>MSLPIRNSIKRYKEQLKKPLFKNEALYQLTKLYLSLENEINENELDECKDYFNQLKQSGVLKESQKELKEITIDFQTITKQYDLAEQSLQSAIKSYPDNLNFLLKNINLLSINKKYYEFFKSIKDSKIKYQRDLKYLNFIIKQIDNVAIKAIKESVEEIQANTMLLNDSMSYLNLITLKTEILDYIIRATIHNNLVSSNSSGSIDDIDDIGDYYGNNNFNQKLTRQLKEFKKQVKKIRELVSLYKEPITLSPSLEEFNERYFFYKGILIDYEYSNISNITTSISNIKNRQNPPFKSYLKSLQKDITKSSSSNMLEPIVKLSSEVSRQLFYSINRIIGDGNEIDLKLNFYASLNNNINMNLNIGDSGMYKYLDYLVSKFNSVSSPNDTDQLDTLFIESIEKNDFQYLLNNPLEFQRFISFSLWHINKTSSYTTLICWLDKIFNKFINRINFELQQLSSKSSSSTTTTTTSSSSHITLLHIIVYCINLIFETDYQQDYQQQQKQQQQQQQQQSYQLSSLEVYLDSTLNVPFLRNSLPWKIWNSMIYYSNLKPSSKINSTEIFSITTLSELLNGILKNGDHLHPLTCYKIAKDLPMITQHYQNEVDLSQTDIDISKIQATYYLITLRHITYLNQQRQQQQQDNNNNNDINNNNNNNNQIIQDKNFLKNIENTCNHCLSDLYKDKQNLKGALQYLLKVDTPIAYVETIYLCRDIIYNNKSNPAYTRPVIQSLITLMNQVWNKCQDFNANDLDYYQVDHDEYLNDIDASLEIITKLKDQYNFYDVPSTPSSSSLYTTPTKPTTVVPFSSIYGNNYNNNNNNNNNSLISSTPQRGRLSLPSTSTPLKVSMLSNSPNKSNNNNNNNNKQIQQSQQNKSDLPKFNVVEEEEEEEEVDINSFKDVFLQRRKERAELLKTLSNKRKALVCPQEFNKPLRSLDYVPPEGTVITKPTVVPTTTTSPIQTNSAFFGTTTPNSLLVNPVVPLPTTSTSPPSLFGVTTTTTTTSPTSLFGKTNTSPSSIFGTTPTSTSTSTAPLFGTSAPTSSLFGTTASSTPSTTATPATPFSTTATSTPSTTTTPATPFSTTATTTPNIFGSTLTTGLFGTKTPTSVSLPQSISTPTLADKTIKTEESTTSVSPPPPPPLPTKSNTPTKPATITPTTSNATSSSSSMSSIFANASVNASSMFGNTSSSSSIFGTPSSQTFGSISSPTSNLGSLFGGTKDFKPVETTTITTATSPPSISENKSTTTSDTNKPVETTTTTTATSPPSISENKPITTSDTNKPVETTTSNTLFGATTTTTGLFGLTKTSNTATGISLFGNSSSILNSSLLSKKDGSSDEDSDEDSDEQDSEEDSEEEKGKTTKSNSSLQRKKNEVSHKKDSKNRLQTLKDKISKKNNNNNTQKDIIKPQQQKQQTSQSSKNLSDDDQDEEYESQEEDENQDDDQANEEYDEDDYEEEDEDYEEDEEDEDEEEEEEEDYKEDPNKPKPTFLFGTSSTTSNPAQTTTPTTSTPTPSSSIFGQPPTSSSVFGSKPTVFGSASSNSSSVFGQTTTKPSTGSSVFGQNSSSVFGQTTTPSSGTGVFGQNSSSVFGQTSTGTGVFGQNSSSIFGQSNGVMGSTSTPSSTSIFGVKKSDELTKKTEESVKKTEESASSTTPSKLIWKCLCCENENSEKEKSCSVCMVPVPKNVKFESPASESNTKPSLIAPTAFGSNVTQTSTPLGKLIWKCLCCETENLEKETSCSVCMVPLPKNVKFESPASESNNKPSSLFAPTAFGGNAPPTTSTAVESSKLFGGGGITFNAPNIFGNNSNPSNLFGSGNNNSSSLFGGNSTTNPPPLFGNKSDVKTEESEKKAEASTPSPSTTSGKLIWKCLCCETENSEKEKSCSVCMVPVPKNVKFESPASESNTKSSLFAPTAFGGNAPPTTSTAVESSRLFGGGGGNGITFNAPNIFGNNNNPSNLFGNGNNNSSSLFGGNSTTNPPPLFGNKSDVKIQESEKKAEESEKKANESTPSPSTSTPSGKLIWKCLCCETENSEKEKSCSVCMVPVPKNVKFESPASESNTKSSLFAPTAFGGNAPPTSTAVDSSKLFGGGGGGSNTITFNAPNIFGNNNNNTSNLFGSGNSTSTPLFGTKPTETKAEVKAESKTESNVEETAPSSTSTPSGKLIWKCLCCETENSEKEKSCSVCMVPLPKNVKFESPASESNTKPSSLFAPTAFGGNAPPTSTAVESSKLFGGGGGNTFNAPNLFGNNNTSNLFGSGNSTSTPLFGTKQTEIKTEVKAESKIESKVEETAPSSTSTPSGKLIWKCLCCETENSEKEKSCSVCMVPLPKNVKFESPASESNTKPSSIFAPTAFGGNAPPTTSTAVDSSKLFGGGGSNTITFNAPTLFGNNNNSNPSNLFGSGNNNSSSLFGGNSTTIQPSQSLFGTKSTETKSDDPMSLKEMSNTIQDNDDQNSDSESHEELESGSEEEEEQQQQPKVTLLSSSFTPPSFAPPSFAPSSFAPSSFAPPSFAPPSFAPSSFAPSSFAPPSFAPPKPENTSTPTSSIFGSFSSQPSGGGISAFGPVSSNSSSPFGSGFGSASIPSFGQSQVNPLTINPTSTSPTAVFGGSTTSQFSSSSPAPIFGSTATIKTFGDLSKPSLSNNENKDQTSSSPSKPSPSPSNPTFESINKEKESVEDKNQEKDELKDEKDELKDENEKKDENEKKEETVESDKEKEKEETLEETKQSIESDKKEEKKEEKLEEIVQSDKEKEKEETLEETKQSIESDKKEDEKEEKLEEIVESDKEKEKEETLEETKQSIESDKKEDEKEEKLEEIVQSDKEKEKEETLEEIKQSIESESDKKEDEMEKVFSRIEETIKPNFFSTKEDEEEKGDELKDEKDENENEIESDNEKEKEETLEETKQSIESDKKEDEKEETLEEIVQSDKEKEKEETLEETKQPIETDKKEDEKENETEPEKHIDNEKKDENEKKNEDEKKEEETVESDQEKEKEETKQSIESESDKKEDEMEKEFSRIEETIKPNFFSTNKDEKDQETKEDNGNSDNNIDQETKENEKASKEIQDEEEEKEKEQEEPNLSLLSMDPVRCMSLSGLPIFDQTVKVEEEIEYEKDDGDDDDDDETIEKDSSSTTTSTTTTSTTTASTLTPQKPLFAPSSFAPPSFSLPTPTIQASSIFGSFSSQPSGGGISAFGPVSSNSSSSPFGSAFGSSFGSTTIPSFGQSQVNPLTINPTSTSPTPVFGGSTTSQFSSSSPAPIFGSTATIKTFGDLSKSSSSNNENKDQPSSSPSPSKPTSESTTKEEKVDIVEDKTDKIEENKEDSEDEKVITEDTNNQSEIKVEENKEENKEENKEENKEENKEEEKEEEKRIKQQQQSIESESDKRENEMEDKFSKIEELVKPDFIPCKVEEKLSEEQTKENIDNNDDNNTTSSIVVQENTTETISENDNDQSIQLDSNKQEIKKSIESESDKKEEVMEKNFTEIENLVKPNLMNSTQEEQQNQENKVEKEEENVNKTEEKEEDENLEKQNQTIEKENEEISELKDIQENNENNEESSTSSDGEESKSIKDVDTSYDDVD[2x];>[8x]MIIINKNNDKKSLFLLLVSLIFVLFVSNVIADTDYAISPVSLLLPYSTSKYRKPYKLEANKGCFEWINTNPDLVEITPLYESAASCSPSSNDKQQNIGAPDLSLWDNSLNQPNKKCSKAVLVSVRSGTVSERNSAFIYAEEQVTGKKLQCEVFVDRISSIVIETTTKTMYKDDLEELHVRAYDSVGNVFSSIIGLEFEWSITSGNIIQIVPFRGFPLDDVALKMEQESLQTSFVLVQGVDTGRTEINTKLTEPTYKDIQHSTTISILEPLQLNPSYLLYVIPGTQIQYQLLTKKRNILENIPLPNPNYIWSSSNSKVGKVDNSGNFMALDLGRTDLKVQHKNMSDNKVQAFVNVVHPSYLAIKIEPLKSGLGPVSNWNLIENRDYILVVELYDASGHKIHSSEITFDLNIPTEYFERLPSSQIPPNTPKRSDTFYLKAIKQGLVALKASLVKVYDLNLKKYTQLLNPISVEQEVTIHSQIQLSPPIVYLPYLPNHRQYSMIRPIGGSGEYNWYTNNSAIVTVDPTGAITSQTSSGQTEVIVVDKKNPHNRDKVLVIVLQPDEIIITPSQVEVQVGQTLKLSTQLLSKQLSKGVHFDSCNLDDLEWRVDDSNANNDNNGGGGSNQERSFSLLPLQKTNTPKKEQPDLCSTREFLAIKEGSNVISVSYMGMRAKILIFAYPPLKSDQSEILLTLGSTLNVFFSGGPEPWHLERKSHFQSIVSNLTNEQNVLSIVPGNGNSFRVTCLTHTNPSKPIGIELTIGNKVTTTNPYPASPSITIPYSCRPPASIQLQVANLPKDHQIQDSSHHQQIQQQEQQQQQQQQQSTCQDTIFSIKKQKQGEIGTYKIRNDRDIPFIAQVFDDNGKPFTNYSSLVFDWKSSDQTQAKWLRDYNQNDHLSTLSLSKEQGKVIITVSILGYDQELLRQNKIRSSDLDTSKLVSSLELHLLSSVVLFPDYYTMYLNDKNHLKIEAIGGSKNFAFTSNNSKIASLSYQPNSDFVTVIPNQQGYLKVEVRDICLGSDNNKDQQQQYQQKQQKHQQQQQSNTSPSIVQISEVHSIELDVQDMVQVGDSINLIVKGFSQNGQQFDSTQYQYMNIIPHIDNPNVLSMTQSSDSQVFTLKGLDQGLVTLSVTIQNPKTSFSATSKTIQIQVFPPFRVSPSVLHLVPGGHFQIHWTGGAPIRQDVSFVSSDPSIVNLSGREDLVGELVALKVGEATIKAIAQIVDPITGKKTIIGEDKLMVYVKNMTGIRIHSSINKILVGNEAKLRVVGANGETPFTYGTVDLFFKWECLDSNIATLLPIYERANTTVEAEGSFSVRVMGKNAGSTSITVWAYSGGDKTKHLFQAASLQINVIPDIPIQTTSLLLPLNTPSSFIVNNHLDKTGIEFYPLMDGHGSSSCKDVIDIGDNKIVSLDKIGTCYVSAVRDGRMDTSKLFKINSKPFSHLELLPINPTSTVIPIGGSMSFAIYLRDDIGEVFTEYGSSAIFSSEVSNTGIISSSIDANVVTIKGIRAGLVTLHVYLKDMPHLDDYIKIFVGRLVEPHQPILHVGSMITFSIAKDQLEQRGFSLPSSDEKVWSSGDPSILQVDPITGKATAIAAGTTTINYIRNPSSQTQVVISKIGRIKVDFSDQIINNSKKRYEYNLKFFTAGSDIELSQDSTIDQNIKGICTIKESTFATAFFEKVKGKEQYRCVVQPSGVATSSIDKVTLYVEVSNAHKTYQYDTTINLPFESTFSIINVRDNKIQLSPRQSTFILNIQSSSPIFVESSDNSLLSVQQISSSGGDDQLNNLYKYAIQPMSVSTSFQNVPLLISSADGKSKTTVTVSYSKSGSTTSDQNTSYVESSTINSHPFLFSFIIIVGTLLIGLYASKKHNDKPRVYINPNSNLQTSSISSPYRTPPPHSFTSPNRSTYGSSSIYLNN;>MIEEHNCFEEFINTAAIGEQQVYGEYKSKLDSFTDESKLPYELLLERKNLVELKISDEEYKKSESALKTPNPTLLQKFQINFYQTIESINQVFKPSSSSSNQSSSSSSSNEDDSLQNKKIKVMSWHPQHRLLAVCNKNDVIYIYYFPNQDMYGMGNVRPLTLWFELQSKVYDIQWKPFLPYTLAVACENGIILWEIDISDLKVELKRTSPNYRINQSSTCANILNYPYFLSNTITWSSNGLQLACGSTNHSSILLWDVVSRVPTFIPRYNGNSLLVWSPKNDYLLSCGGKTCRIFDISKWDYNNKEWPMLTNYQTGSWNGKGEYLAVASGDRIQFIQCINRAFESGGELMYVEKTSTYRLQNVGGSGGGSSSSELFLGGHIKKIAWSPDSQRLAVIFYLNSKSRNNDTYCAIYKIKTYPKFSVTPRGFIRSKDQSIQSVSFVPNYKKGSLLSIAYNDGTIKFFPLLYQYKQ[2x];>[6x]MNVKEMDFNDLSNKSNQIINRISSFSSPIGLSSFNIERNLQEIGDTSKQLNDLTSSKTPFSNPLEPNVFQDSKINRKYGLDPKVLAKNLSNINTSSFTDVQSVPTDIDGYLKVQFENIILNTICDIQKKTSKEFQSHYEQTSIHDWNRDKKYLEEILGQKHIKVLPSVGGASASNQSSSSSSLFQQSVRGGLSSSIMGQSVRPTYGQQSQFGGSSTISIGGNISRVGGGSGGGIYSQRQTGQNEDRTKLSDKMKKYASIIEEYDIHMADQSKSYGFPLVHRLMDACLSTDINIGGGINTNTATTIVTHVWNLLLTLTSEIDTTNYIQQLKEQQQQQQQQTPQLKEQQQKQQQLTELQKHTKYHTKPTMAQLLKRSISFLETQFSQVIESRLPKHSNVSLPLNIIVAYIKSLNQSPLTDSSDEIYEGCSIWCIIYYLLRSGYTLEAYQFALEKCGSRYFDILSPIFKEKQQQQQQQQQQQQQQQQQQQQKSSLPTTTNNTSINKDQRDRMTREFNTAKTESKDVFKISVFNLLSCNDPNSTKQQVITSIQDYIWWRLNFIRERITIEPTNDSAISLLESLQNDIKNSIEKNRNNYETLEIFQLLLVSLQFEDAIVSLYQFCPDDSLHLAIALDYYKLLRTSNSGINNKHVDEINKFNKSTTNTNTMTYQQNQQQQQQQQQQQQQEQQKEIYDQTSKSIHLVEMIKQYTKIFSFEENREAFFYYLLIADNDIKIQEISELVVSSPNGFKFAHELSLFSEFINKQQWRTIIEQSALELENKNEYQSAIEFWIMIEEYPRVLEIYNSRISVLLTSISSERDQLYQFGKQLFNDYQGRLKTTSTARTSYLAFEQLLKLCDFFDLYNKEKYQEAIQKIENLEILPISESEIDSKVQDYRFLSPHITRNFSSIIQAYVDIIVKQYHLLNNFDEFTNRSALFAGRKQTIQDLQSRTQCIALFAGKIDFPMSGNILPRLMNLFISMSN;>MSNTGGNGNDNAAPSLSTTTENVNGNDDTPSSNLTINDLGGSKFPPQPKKSKQQQQQNITDRLSTFSNFFEDEKLDKDDMKLEFDKIEKKLCDIFETDTIPNNASKDQITSGKIKIKGEEITISKEAQDFTLELSSLLNLDQILTFILIREYLTNNNNKVLNYDKSELFNLLDYYYNERASLLCILGSIIKKESSQSKYSSFLKPFIEKNRASIESRLLSYLISFYNFTIPSNLEELQQFYCSSIIKEQLIIVETLFSYNYLKVKKSGNCSNSSSNMNDVNELLIILKKINQLQIGSYSDQLIGILNSMKRNSEVIQWLKRIEYVLVLLVFCNNRDLLRHESLQQNELEIINTITTLSQSIHYNAPLATSLFFTIINLFISTSSSSSSSSPSSSSSVNFSNSLQQYFTKASSQYDPIDYIFNCLSNGFNDSTYLAGYCDCIHIFLNRFSEVISLTDVSEQHVDRIIDIYCMLHEKGGEVLSSILWSERSNDPVYQFSISPDCLNRNPDRVLSILKSIIINDTSSQAVFNELILININNQSSSKQIISFNDFNKVKEVLDITNDDGNGTISGVMKRDIISQSFRLYKSQFKSFSVINDGSGGDGGIEIVFTLHDLIIDLVAIEFNSFLDSLGQQAFFDQRTIEVSKAYIVVLDLISKLVNFTPDSYSKYFWQLFENNRILESIIQVYLRLCNQQNFTVNSIPTNINIKESNGNGGFQQKINKQQQQQPTLMSSYSTAHYNFNIITNVITSILSLFTSFSKMNPLPILNLLIEKGIWSSSPTVLISLFKRGSFNHLYDVEKRSSTTSSTSSTSSSSLSSSTFPLTKSIVKLFNTFINPLNQFEKCIDRSQYIGYLESFISFHLQVISDYPIISGNNNHNETWEMISEIFSALDFILNKSQSRNSILKSLAFKIICSFSGGILQCTLSSLLDLEVLQNTNKSIDRTSSIDNILKSSLKFSKSILSTIYLSIVLKRSNKINNNNQNNDNNNENNNNNNNGDNNNNNNNNENNNNNENNDNINDNNIENYENEYSNNLVEQFLTTFFIVKQNETNLLIDQEDRNGLTSTIVTNSITTETITSKTDYNNLFIVLFNYINIISDCQDIQILSCEILSSLVRILRVLESNFSVSTLFNTDEPFILMIEKFSKKFIINNNEFDVWSLQLKTNILRLLVESSTNQIYFINRLLNCENNNINNNNNNNDDSGGDKKNKSFIIKLLLDRNVSINDNSEFSLALFQLVNNLYCNSIYYDSFVDQLNNTQDFWNLLLDMQKTINEEEEQEEESIINEELICKKLKITYAIEILSLSVLLSSDITTATTTVGNLVCSTLSNNKWNEIFKNNKSGIVNMINNYYFQFIDLENVFPIQKIRDYWMVNNLPSPDQLQTTIAYQYFPNINNNIPIVELFAIDTIIETSKQFNDQYYLELLIQRNLFELLTTTNLCLSRAFSKLFRVILMKQPQNFININGGSGSGSGSSNSGVPLSTILHTLVDKATSIENQSIKTLVVRNDILMFLCESISTASHLWCKSCPIESVDIEILSKLSNLLAQCSSNPILGHSISYHILTSILILVENTSQHQYIEIKVFNQLINTLSLFITEPHFRVPPISSMDGTTTTTTSGGNVGEGKTINGKQKKPLPSICNLSIYLLQVLIDRLDPNALIAAFPNNLLENLAKLLKNSLNMVNGNQIDNITASSVLNLLISFCKQPLVSEQLLDNRIIQLLSDHSLKYLQFSMDPYLASTEISAATASIYGGINYYFHNNDDDYDNHRQFNQKKNKWHRVWTLVIKFLISVSKPLESSERFIEQLSNFILSHKDRLFYYFDLFNEFGATQHSQYFTKQWFQQLEYITSLFSIFTKYTKRYYLSMNIYREFLSLAYRLLVSISIQCSELNFIENNFIPITKNEKHKNLVQVKEFIDDSQRLQQQQLQQQQQLQQSQLQQSTPYRTSHYQQQLLQLQQQLQKQQQPQQQNIQNSFFKFSIESNYTHIINNCFTILIRINEYVRSSNEFVPQLTIYPNVATFGTFGQLSQYIISKLFQISNVVDKLSRNNNNNNNNNNNNNSSSIYNNLEDQNSISVDELLDLNLYKTKIKQTLEKNTLLLILYAKQTPPSTSPQETLRENQVNNIITHLLKQQFNNNNNNNNFSQNRTPLKNNNNNLNNNNTSENDENDEFLNFLSDLQRVK[2x];>MEFINSFNLVMSNIFDNHNNSSIEFWRICEQINYFQNLWFRIHDDLIISSFKLMGSLARCNTNEVFNFFAQGSAQFTWAKLFQNFSSYAHALNSIEFSQSIQSNQMNSSTTTTQQISSTPQQHQQHQQQQQQQQGYNNQQIPNTPYQQFQPTMQYQGQQSSMQQSVGQQQQPQQQPQQQNTPNTPNSTTSSNTANTTSPVKITQLLLSEKDSDALSSIFQLISRLVESSMAVGNVFLKIGPLISLAFQFAVSQVDSKLKSSALSVITSYSQYPIYVADIWRLINETNLFNSGLSAIGGLNELSFTQQSLELLLQLIQQSSFLFDKSNHYQESLKLKSYLDSCMDLFNLLNIKSFNTLDEKWKFALTLMKIFEFSIIQFNQSIQNFQIDKQHPCYQLYIELNRSSLSSNLYQQQQQQQNKYQQQQQQQQQSKKTTLENIIKIIDYSNDQSILIQQQIQQQQQQQQQGYNQDSSRVILNLVFQQLQQQDNDDFNLLVLKCLDLLLLISDNTVYDIENAKSLVVNLSNMDYSRPIVSIAKLIDHELPAISLRAIRLIYSFECYTHQISTVFLDSDPNLILSKFIKMMEFNESNFEDFSGTNYDQTISFIRYASNSVQWTIAQLIMLCLSNISSGRYTLAHFLLGCSSNLDLSKDFIPNSKSCLTLIIKNVMNSQFVERYPHLVDCYHEIIWKMSSDPITWKPMIKYIQEEFPNYYHDSLLILRNAITINGSSERRTEALISSMSWVFKTCSISIQNSYSIEMKQFLTRLIFPSLMNLNQPSMNGGIGGLNGTINNGLIMGISPINILSLYNTIEFQLPEINRPRIFSMYPNLIEYFTTNININNLNSNNNNNNNNNNNNNNNNNNNNNNNNNNNNNNNNNNNNNNNNITNGGTSQLLDIIKIREVLKNDFNRFSNEFEIERELEECCLINSSIQLYNSKLKALDGWKSFINISLAQNTIEIDTLDESLLLSLLQRIVIDFSNERNPIESTLSIGYTILTILFTLKLKKDSYQLFINSSLTTNSTDSNVIEQKMKSIFEGLLQTVLKSPHQAIRGISYTCLIQYLDLSATTPTTPSLSPLSTSINNVVEMNNKSKNKNNQDKEQGYGNLNIGLIISKIEDKFIRILSSDCNSFSRGWRITAISCMQSILSIDNLCGHRSLMFLQNKGFIINMINDTCSKYLSDNWENIDPKDLHVYKSQMSLLLKISQQMDGVHLLMNNNVIGSFVKSPFLNYIPTDKIFGKFIEILLPILQLFASLCCYCNNTSKNNGNINNNNNVGGTVLIGSDRNEIYQELFDFLSNHSDLFIIILSDQSSFSHPTLSSLKVLKLTCFLFSKVSSLFFKKSTTTSSSTSTTSSHNRTQFNRFHYCLINLLVKYSVNSKQIIELVKPENIDEELLTEKIDFSYLPKSSIENQFKNIPDDINIGGVNIGLTSKNSNNNNNNNNNNNGSINGKKSKRKNQFQILIKETITSIIHDLLLYCRKVSIVQDSNFGFVCFNSNLNIYQQFQSFSSLRSTNRNNSNNNNINNNNNNNSNNNYNNNSMNSDMDNDDDNIINNNSYKFNNKNNNNNNDNNNQNKNSIFGGFGVNNSIINGNNNNNNGNNNNNNGNNGVNILPSIDLAINILVDNILQYSFYKVDLSQCFKLLQSYDQLTNYQYQEILQTGEDYPAFGPTQRNHMVENILKEKIIDIETQISIIHENIEILLLLIVSHSFYFCNSLYLLFQNSNNNFYSSAIGGTISPTLASSAYYPTTQQQQQQQQQGGSNLKITDLNASTTTSNIKKNNESAFLSSKTNQNSGGMLSSVFSYFKGQQNNTPSAQVSQIPINSTPYSTNYATPHQHQQLLQQQQQRQQQIQQQINQTPSNELSPQEIEVFLKRLKQSIFEREVNQLGGKLSDVILNQIDKKSTLIDLLLKKLQDLTK[4x];>[4x]MRQSQLYPNLGYNNQNGQFNYLPSPEQQSIYRNNIQTPTSGISNNLFPLQSQQRIIQPQYHYQTPLINNNIINNNNNINNNNIVYQQDQQTQPQAQPQQQPQQTQTQSPSQQEKEQEQQQQELKEQQQKQQQQQEQEQQELMRQKKTNSLLSITPFNKEEDLKKIFLNSIESIDSSIDKVATIPDPTLKVLYKRDPGFNYFDGGSYFWSTLVIEKHIELPQEITNGYLSTSTKSLLGLFPEIGRAWISIDQTLYLWDYRDSGELISHNLSQIITNCALIQPKKNTFKDAVKKVMVVCTHVEIFLFALCYSNETKFEILSTLSIPSDNIFITDIVGTKEGRIFLSGQDGNIYEIEYSKDNLFWFSNEKIKKINLTQTFFNSFINLSKKKEIIQLIYDEDRYLLYSLSKDSTINVYSLGKIGDKFEHLKTIYPINDIDSLFNNNINNNNNNNNYYSQQYQYQQQQQNQQYQQSQYGQQQQQQQPNQYGQQQQQQQPLQQQQQQQQQQQQNFSRKNMVIMSIHISPKETEFNFIAILSSGERLYYTLNRLAYIRSPPNNVDNNGNSNIHYTYYSNGVFFTASEVSDQEDRLVGTTLFGNDIIKSHYETSKSGFSNQISQDTLSEKSNLFSIRGRVSVIKEDIVNDGKPTVYYKELSNEHMNTPRRFLCLNSLGLHFISKLRYVDLLQNILSSNNPQDIDNFFDAFGKIIASSLCISLYCSSPHSSILLHDQVYSGISIPKTTTTRIADLAMTFLRRKSGKPQYYQPVVIQQMFGDMGAPVNKTELMYSNAYNGLLAYLARVLYPLWNQSVVTSAGCSYWSIVQLQLFQSHLSNLLSFLDISQLIPKGQEIPIIKIATNKTSSTTTTTTTANNSSSNEIYGEDEAIKNEKRSLIGLKNIIVKSIQILNLFLILSQYNFKQLFDSSSIELDIKRKIDLLKFRDILNSDILGKNLPLPTISSLTTSTTTTTTTTTTSTTSSSSSSTSPLTTSTSNSTLTLLIDSLMKTLNSHNINIDQVSNQLETECPIFFKKENRELYKVKEKLNMVLRDGSTYFTDSLVKDSALILDSISPNYNLSEIVDLFIAIKAFNYVTPLCLQYAQDLDPRGITLIPSNNPSDEFKLKLSQKKSTFQEIIKLLNFIQSDNNNNNNNSGGGGGDNNNYNNTFEIIDIIIQQVLVCQDRLAHEMIYSWILNNGMTSKFFEINTPFITEFLFANDIDLCWKVLAKHQELLKAVHVLFQIAERSTTLDEKILAYTNCTMILSEQKDEDAYIQAKNQITFANIQKQIVLQLENYLNNPNESNNRNNSSNNNGGQPFDINQIKESISNLNKTIFDITTLFTDYARKYYLHEQMLYLCHIGNHSDQNFIQILWKIIIDKEIPPPSSNLSLDDNAENDDGLKISVGGVIESLVSKISNIGYDFYPNEITFPVEFIINYGERAIFNFSRNKSEAEKKEISPNWLTSSLHDHVKIDYWILVDYYNNTIEKGSWKEEDESLIYITSVYFYLVESLINTIQTATERRLFSSKQILQSLENRESTFKSIFNRQRSSLNQETIKKLEQLLIKFEKIISISKSFKDFRGY;>MQSQPQQLQQQQLQQQQLLQQSQLLQPQYFEKQQIADYIDKTFEKKIKEWKTWTFSSVFIIFLPLLLFQMLFLSFMFSPSPKSTSTSMISVILRTTGNHIFGIILYVIGQLILGASYHSICSVYRQVPASFKEQFTVLSIPHLIFITLNTLIQPLFLYFFFSIPLNKFSLSSIIEVCYQDFSETIPVAKCELEYNLFFYLFVLSCIGLVCSGLFRIYSNQEFVYSFPKANIPTFIQIKSMLYNNFWISFYTSFYLFFLGSFLLGILFLILFKTFTIQILIFSIKLWCFTFAIIFQNLTRNRLFEIYFTRGLRFTLETFNSVTFDSSNSQQQQQQQQQPQQQQQQQQQTLFDNKPIIENGSIFLLKAIYSCDPLIQALGWKDFLHLSKYSQPRRTYLYREMSELLDQPSILKIIRQYEDQINDLSLKLSCPREYYESLNSGNIKKEDDKNKNSNNNNNNNNNNNNNNNNNNNNNNSNNNNNSIIFKIGNNIEKIIKKTLNFISGVKFDYNLYECEIRQALSNTQSILWSIESIGSLIVSAQINDDRETMELLHRYQIPQKFLIPLFQILALIDQLEKDLSHQIELDKFTINRDYYFLKSFSNLIEPPLNCLGILKTSRPHFRIFKLVGKNMISQVLETIGHQISDISFPYDLRTTLNSYRNGEFSIYQ[2x];>[4x]NDLLSIPVNSIYEEKYDKRWLTVFGFSHDKTDLIVDELSKYGNIIEIEYPQQPNCNWIYLKFESEYSSIDLLKKNGLILGNCMIGIVPCKEKIRN;>MSLFGNTTTGGGGLFGNTTTPTQTTGGGLFGNTTTGGGLFGNTATPTTGGGGLFGNTATPTLTTGGGGGLFGNTTAPTTGGGGLFGNTPTQTTGGGLFGNTATGGGGLFGNTQQQQQQQQQQQQQQQQQQQQQPSTSLFSQSSLGSQSSLGSQSSLGSQSSLGSQSSLGSFGQTQQPQTSSLFGNLQQQQQLQQPQRSIIEQKLYDFMQSISPNSLNCRFLYWFYNYQANGQLVDPNSIPKPPNVTVDQWAYALSNNPDPSILIPVAAKSFDDLINRRMKQEETIIALDQNTQEALKRMRDLENHLNFHIHTQLEMMRKKQIELIQRYIEVWSNLEIYQSKGKTFTTSEERIMKKIYELFEEINQPNSIKSKVEEISNQLKLGSMEKEKIKYEISPEAVEPLYNLLKNMTISIERITNELEIAVKDAQILKNELYQLKKC[4x];>MFQTSGLFGQASTTTGGGLFGTAVTPTSTGGSGLFGTSTSIAPTSTGGGLFGTSTAVTPTSTGGGGLFGTSTAVAPTSTGGGGLFGGGGGGGLTSSIGPQGGGGLFGSTTLPTSTSGSGLFGGQSSIGFGQPNSGSGSVSGGLFGSTSVQQPQQQQQQPQQPLITESTKFSDLPPQLKNELQILNKMIINNNSLMNSFSNYDTKINEISIGLDQVASVMDNLFNNFDIHIQSFKYLEESLAKPLNSVNEQVHLLSTQFHSPFSQARPSKEMEIIVDSLVEKIDRIKQTILCVTPTNKSQSQNLSFQESFISTLQSNQIILRNLAYIVDNLVTELERHKKHFLLYKKKYYNQNYNPFLKQPKLNEKTDYHGSSSLHHSHFSQSSNLLSSQSSLFGSSMYGRQSQQQQQQQNPQQSQYLQSSTFQPIQTSTSFFNPTSTTTTTSFGLTNNNNNNNSLASNNSSGGSSGSSLGSLGSLGSGSGSGLFGSTATNNSLGSTSSSGSTSSSIGGSNSIVIPPLAIGSITNNNSGGGLFGSSNSSSNSLNSLSTSSSNLFGPPQTPTLSGQGSTLGSVVFQSLVQLQI[4x];>MSNNLFGTGSSTSSSLFGSTPSAGGLFGGGSSTTPATGGGGLFGGASTTPATGGGLFGGASTTPATGGGLFGGASTTPATGGGGLFGGSSTTAPATGGGGLFGGSTTTAPATTGGLFGGSSTTAPSTTTGGLFGGSSTTTPSITTTGGLFGGASTTAPSTTTGGLFGATTPATTATTTTGGLFGGSTTTPSLTSGGGLFGATTPAATTTTTSSAIPSLTSGGGLFGGSTTTPSLTSGGLFGATTPAATTTTSTTTPSLTSGGLFGATTPSTTGGLFGASTTTTTTPSTTSTTTPSTTTGGLFGATTPATTTTSGGLFGASTTTPSTTGGLFGVSTTTPSTTSATTPTTTTTGGLFGAATTSATTPSTTTTTTTTTPTTGLFGSSTTPSTTTSGGLFGSSTTPSTTTTTTTATTPTTGGLFGSSTTPSTTTTSGGLFGSSATPSTTSSGGLFGATTTSATTTTTTPTTTSGGLFGTSSTTTTTTTPAAVAATSSNPLTTSMLGGSSTTPNPVSASLNNSDPIGINESKLLEQLLNEWVSEIENQTKNFYDQAKTIFVWDQRIMDNSQKLGKLMDVVVKLNSQQNALNQCIDVVRDQQALLERSLNALDSKIKSSPKDNETTADLERERIYSLATKIDDDIIKVENKLLGVVNKINQNQVKDDNPKDLNQKVSKILNDHLNTLQWIDKSTNILQESLKVIESTSLPETSRR[6x];>MYYSSSKPIKKKPNTGISEFNPTQSQIQQQSCNYKITPTYDLPFILTQAINDENQQHQIEQDLTGSLSSRDGTCFIIYSNELFIWTIDKPQYCDRIELPIKQNITRQHIVVYKNKSSSERFSVFLCSPLTGYIRFWGNSSKPNVSQDLPLENPGNNNNFKIFITECQPFGVIVGNSLGSIYLVSVKNNNNLISKKINKSQGMLSYLYLSRQSPVISVFSSPINQQQLQNNNNSHHHHHHHSTTLSSNNFSTIPSRFIYILTEGSLLKYEIENGTERIILDFPIQKEITKLFSNFPKFHQMNIDTIIDQNKDEIQIVNFILYETSASQNLVKYYILQIEIQDDQVLRIKRLDSFSANKKLGGGVTSIEPILQTNSLKYYLTWFDNIYYYSNGGGGGGGVNGIISGSISFQSDIAFSGFYKNQFYFFSEQGINKLDIQPFGSGQLASSELHIQDTIKNIESDIYMDTDNTTSVTGTPATTASATISTTPTIVSPILFDIPKDENLIGSKRNNVLKLMNSFSLKQHTRVDQFVKICKGYNDFDQVIQQVSLWIIDQQPNSKFWAEDGKLLHMFVKEISVQLNQQLEDKKKRHNFLLTCIKDTDLDKLLTTQTKEILKKNEIKIKCAIELRNYQNQQEQSRKSLNYTTTTTTIMKGASSSSSIFSQLIESLVAERNPNWTNIGMNVFELFYSNVSGIDQILINITSKLQELLQNQPQQQQLLTSANKAQILLENCELFYLISSSFPVEYLNSPIIQSTSISIHNLFPKVIQSILNFIQLEFPNQVAGLLGGGGIGGLGNGHSSSSSTILFKKDLGIPNVDKQLYDHLYKLTEKYLYSLKINQFEQFNQFKTKLIEPFVECFKFQEAITLANQFDDFFTLINVYCYQQHQLQNSTITIATTITPADNNKLLIDCLNKFEKIGQLSKVYEYMLERDLKSELLQLPSDFNDSLFRFLQSNSELSWIHSIRMKNWTNVSNTLYQKSISNQHHQQQQQQQQHQVMTLKEKQKLLSLSKVSLMVSTATSSSSSSSSLELQLQPSQQIQLDVINQNLSLIKSQKFFLPDLKNVLSVSEVVQLILQREIGDEDPMVNFVSCIEIISESPLLLKKEEVKELLKLILELSIVNETVFFEKSISDIQLSYSLKETKFYNLISHPHFPKEIALVLLSPIIEDFYKTHINSNKFSSLDDKRQFEISVARLLELSKLEIGQKQI[4x];>[4x]MSENFKWNLGNNLNSNNNDDFFSTQPFNNNNKFDFSILPDDNNEDEFSGIVNNNNNMNNNNTLVKGDGGIFGNTQINFNNNNNNNNQFGNSLFGNTINNNNNNMEVNNDNDNNNNEQEFEMDNQQLQNNQMEMEEDENQFNNIFNDKSRTDDTIYHNTLEYELQPKLNDDPHLIPIELSDTFLKLSQAKINSINDDESNKLFYMQNNRKQKEQQLKNYQMEKDTWSILKKLYEYRDIQRSIDQKEKIDISQPNQVQVYNYLIKKDHKLRENLILLEWLEEMSSQVELNDNDAVFWEYTLIKLKKSNSITMLTNNQMVSELDPDAMSRQNKPIDKDDEKNQSRFLKTVWSFLRAGDRVGAAEYCTNVGQFWRAQTLIGLNYYQGEHSIGNPYFNLWKSNCLNISKNSNDQYERAIYGLLCGNLEATLPIQKNWYDYFWCYLRVLYDESLYRELKPYRSPLSIEEDIDSPPSTCISQINTPKDILEILKNNTSQIEIKNQSENPYHQIQELIIADDYSILFNSLPNLLLKNKTPEFNRFAVLLILFFRKREQYELISTSEDCPENIVINEYVQHLINSQQYELVALYTSLLNNESLQVDVYSRFLVNIIDPNQRQQLLVLAEKFGLNTQEIAQSVVKTITSGSINTTSNSFENLEFTGFATTINKNKQPKNKSTTTTKASTTETTTNTNTTTTPNLTNTIINQDSSITTQDDLVKINSIQWLCFEKQLLIKAILQSNLLLRDFISLNKYGAASELLKSLPKDIVMIAKQQSPLNESDTNNIIKEFRDWENYITANIRINLWLQNYSNQPKISNYLPQSLNNNNNYINNNNNSFNNIINNSIINSSIAFRLRGNESYAEKLDIERRKKEYDDVYGQWNQNNINFGKEAIVSIRSIIKTGWLCPLENQIGLFSEDDQSGHEVTLIRKKCIPSLFKSLYTILVGIGSIQKSSQLCNQIANERFRWYSIFSKKELQEILQLVRESSIKLLN;>SKYSAPDFDEDDQQMQQQTQQKQQQTQPSKVTFQQPSTKLTKPKFTANLDNFDSDSETSSGDENQDEMVPQKKTPFIKRVSNRESGLFDTPSVVPMSE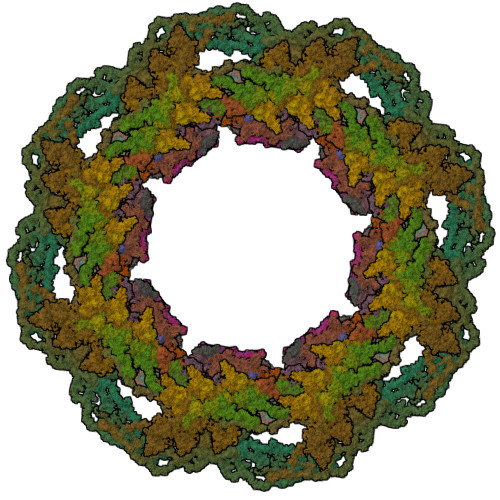KIETTPSKIARVSEPTSQSSRMSNNALKFSTFNPQQQQLQSSRFKSTGLSILSNPVKNLIQSDVNNEQSMFSNTTTTSTTRIQPLPSQQHLVQPIPTTISLNKNYFSKVRIDPQVYDRIVPKEESITNQYRMKNERLNHSTQDVSLFMRRSFRVGWAPGGKLISITKSSFKNLLIKKLPTDTKEDKKESIIKFLKNHHSHSSLVPENLKSIGWFSISNVQEQIESQLTLNVPSSQSVYYNRIWSLISNLWGNVLKGNGSKYINTNYSEDTIRKLNLNQWLKDVIAPLLRDEMDSLRKKTNSNYLEQIFSYLSAKQIKEASDLANENKDFRLATMMSQIWSSSESGKELILKQLTTYHSNGSDEFINEKRLEILHLIAGSVNKIYKNLNDWIRCFAVSFWFKYSLEYSIEDSVENFERSFNAHRSVYPLPPYLIKSTSTNSKQIEEQQHYYDICFLLLKLFAVNRGSSHFDKFKNIFYPENIGQDLLDYHLSWNLYTVLKSIPSLNKQPDLVNASNLHSSFALQLERLGLWQWSIYVLLHTPDQSNHVREEAVKSLIARAAPVITSEDRVFLTTKLHIPEIWIDEAKAWYSGYDCNNDIYDQIDALFKSYQYTKIHDIIFSNIGPNYIIQKRYHSLKDLLIRLEPHSSFISTWRYGGSIFLEFADICIQYKEILSQLSNTAEEIQRTKYYVNLKDITTRIVNILSDISKITQSSEIKNTSASYKQSLSFMSEALITKASLLRDLPESIVKLVSTNNLVSTLNSLPLTQDYRSKNLESLTDQIQDTLLNSIYQ[4x];>[4x]MATQNVDSGHEDMVHDAQFDYYGKFLATCSSDKMIKIFDVGGENPQHLVDLRGHEGPVWQVAWAHPKFGKILASASYDRKVIVWKEVGNNSWSIIHQYAGHELSVNSISWAPHEFGLSLACASSDGSVTIHNYNNNVWEAPQKIQVSQIGVNSVSWSPAAIPTSLVNSANTIIPAPIKRIVTGSCDNLIKIFKNVEDKWILDKQLEDHKDWVRDVAWAPNIGLPYSKIASCSQDRSVIVWTQDENGVWSGKPLPKFDDIVWRVSWSVIGNILAVSCGDNQVTLWKEGVDSEWKLISHVENN;>[4x]MRVFHRLSTAHDDLIHDVSYDFYGKRLATCSSDQKIKVWDQNDNQKWELSAEWKAHSGSVWKLAWAHPEYGQVIASCSFDRTVCIWEESEDEKGQKKWQLKAHLVDSRDSVTDIKFAPKSFGLRLATCSSDGYIRIYEAMDIMNLSQWTIVEEFESQKGTSNCISWNPSSYDKPMIAVGSNEPYIKIWEYSETARKWLQIDTLTAYPIGSTISSSNLNSGGGIGGGIGSGIGGGIGGGIGGAGGSIGGVSGVNNSSMGNLGSGIGNNINNSNINNISVGVGSGVGGGVGSGVGGSLNNGLNSAQGNSIGNGNIGSLNNISGNSGGLNSNSLMSGANSSINVSSGNNSIYSNNNFDSSSDGGSRAIHDVCWAPNMGRSYHLIATASKDHKVRIWKLSSDKSKMELKEVMRKDDHKSEVWRVEWNITGTILASSGDDGNVCLWKCNMNGEWKLFSLISGEESTEDKYDR;>[4x]MFSLNPQSNGNSNNLFGNVTLGNFSNNSNNLFGGSSTTSTNTNNSNNLFGGSSTTNSNNLFGSGGSSTTNNNNFNSNFNNNNIKNENKIKNGKKFYNFRWSPTGEILLYNTLNNFDNHNFDQKNGGSDTIRYEMNTTLSTIKKFYNDLYTNFETMQRIAGLSNQVIPDDRVREISHHSRTYLSVILAAINQMSKSQKTGSYIDDEDSCMNCDPLDNDLIKIQTPRVLEYFKQYPNKTLIFFCGSIDSIYPYLCSKLSMETKSKCILIARESNVPNSKRLDLIRTISNQGELKILNKDEYSNRYQIANENYGELDDVLTLEIDDTYLAYEREIDNLICMSTMWRVANLFYFSVSSSSNSVSPTQLLDCIELERKELLNSIEQQGTQDPMDSEYYNQIARLLVCGCIDQVIQQLNILSRAPRSASQIKSTSRKSPINLLIDILSSIPLKKKSINGGGGAPLYPNEHLIQWNKWHQETQKILSQYIESGSSSTNQVDENLLPIVKILLGDQQTIMSTCNSFLQLVVSNILFVEYTTSTTQLRQLFTQCYQTIQAPTTVDKIFLSFATKDLDITLKKIFKHSPAWLAVHLSDLLYHHPYVMRKLPNSESQLTNIREYLLSDFGQSLASDSSLLSIGCNYLKYVKNGGLEMIDQFISRQPIHFEKNAIKMLDKWATSVETKNSIYKMLSLQDFKRKRYAASLNWLMLANDNSHITLLSNYLLENQLNSEFLNDLQSLLEKNDEIDCNINNNNNNNNNNNSNNRISGNNNNNMIIDENKFEITNNSELIFLIRYRELISLWKERSFKEYSSSLCLMFKDRVIPKRFWLRLLIDCVPLLESLKNLYFTYQDTLLLQSCLEEIIQSHLFDQYSFNISNQDIQILRSALARNLAKSIIS;>[4x]MSSVSVHYSTHKINKVRFLNRNFHNDTSLFVTGTNHPVLSKNKISVWGLESRQNSDEIEELASVPIDGIVTELKVIEINNKPMIIGSTSKGSIFMYSIFNLPNKFEYIGYDGLLDKKYENYNNINNINDTYDTCNLLKERIWFNSSSNNNNVNSNNINNNNYNNNNNNYNNNNNNNNNNNNNNNNNNNNGSCINSFDISYDQHSLVTVGNDGVMNLLSIENLIPIYTNRYIDGLSVNVVKSITSNQIITSGELGRYIKFWDIRSNSSQPVKTIKTQCPRIFSLAIHKDEQHIIAAGSSDGQVNLFDIRNDYSIDQNKTHNSNVWELSFSKSNPNQLYSCSEDGFIYQYSYNKDNLGGGGMMTLPNQINNTFDIYSKEVSLLQLPTSIGSIDSFDINSNINRLICCSTSSQCLIVKSL;>[4x]MSDNTMNTEEIENENGFDIINDFNKVLKYNEISLKSFSDHSSNQWREFTIDSNSQGYYGYSNNNDINFIQDKFTSTPYRSGGFNYKKSPLTDGRFIIWRLVNKSSTLELCEHYSHHSLESNQIRIHFNNTSIIGDVFIQELNDYVIIMVTTISKTIYRFLLPHPSIIEHSDSRVGIKRKVEVDSFGSGSGNNNKRNYKSIFSNLLNSNLDNQWSRVRGVLPDSFEPTVIRYYSATKLIIGSSGSGSTWLELSDIKQSGDITVKKFDCKEGQGFFSSWKWGEKQEPVQDIQFLSTTTNSNNNNNFPLALILLNNSQLKVWSANDKKFIKEITISPENWNNNNNNNNENNNNNNNNIPTSPNINSNQQQQQQQNLSLIHKRFKIYQRSTKSFLLVVYFQFNSESQFQFFSGTNDFSNGINIKEERFAFLKGKGLIDFNIHNGILYSIWSQIKERNYNRGRINRDQEFDEDDNKFDRNHFVDDNNDQEEEVIFKHIYIGDLINFNHQKLSTSNGNGNGNGNNNLENEKEINMEYNQFYNGEMINTFDKYYETIIEHSDEDSDQPTDQTYYYNLLFNRGLFSPNSIEQALNEYKKLKDIDDHGGDNDVEMNNGFDNDNSLESVVSNILNQEDFKFQSNEQWSIFFKLCTKFQKQTCLLGSGLFIEPTSSIIFLIRSNQLSIMKPMKPIECLYTISNNINNSNIISDKQFYNIILNCFGSNSNVLVNDFLYLMKCCNFIDRFIKDDYRSFEYELSRQHVNHTLLKVSEKLIANSYNNSNNNNNNNNNSNNNNIEDNINNYSIGFIKLFKLIENPIETINLILKKFKEEFSNQNDMVIQLQQGYKNIDKGWSGDLFADILTNCFVSTIEIKYQLLTKLSLLLGTVSNLRTHLGIDTKTLFTLEKSILPDSIKLLSTYYLLNWFTKQNFIKSFDNSTTSDIDKILISQNQYGDDSDNNNNINNNEYYEDQQQQQNQQQFTISKNLNILTILINRNLNQFTSKNEFFENIEKQLSKLLCVLAPHMDLFSMGCYLVEKNQYKQLMEFLQIIENNELIEMITPFYYLMGICYAHYSKFNEAYQYLLKATESIENQNQDMLKICSISKEELVCSLFVDIPIDNRMMNQTNANTTQTLISNYYLKCIKIFETRNQPEFIIQFSLFAIDYLTLEKENFSRLDYLNKLESLYSLVFKYSLKIQEYDLAFTASTLNPNQDVSQENKRRLILTLCENSVTTVNNNNNNNNNNNTNNNTNNNNNIGSGNSIKVLCKLPFPQKDIEDNLLKLASAQDLNKKPDYHTILYAYYISRCNYRNASMIYYERSIRVNIEGLGKSRGKSIFDQQQLLDTKLELLSTTINTLKLLDPSDQWIEINSSSLDIRSTNIYNNNSSLNIANHHQHQHQQRKFNYIGNNDEFKDISVVTLKEIEKEYSYYLASKHLCSIDSQINSDFILSPQQLLEKLIQYSLFDVAFSLAITQEIDLGAIFESFASKCVQLQLNPQSNPFFIKNTNGYGSGVIGNGANNNNNNYGFDCSELQHLKDKVTLTWKVLENYLQRYDSDKDFQCLSPSEINENSQNPNTKATIIGNQQMQLRMFGEIQQGSLVDRDCNGCSFRVSDSKGFYLDVHYSHRVPPFFNDTQSGQQVIVIGKLQDGRFIADNVLCKQGQLRYHELVADTILYEGTLDLPTWLIQWFSKGRQDTLFKLYFRHSRLIDASITLRDLFKHAQFELNQINNNNNNNNTIKTSSQITSKTISLNIPYDLIDRFFIEAKKIKSSIIDQKEKQQLTQELTLAENEMIKYFSKVN;>METKINRKLLYPPIDNFNYGNTHHNNNKQPNINHEEIPSGITSDGNYSWFTKENEIFFYDLNNGKRITTFCFVVENSIECSVTAVGEIIVEDQIFIVVALKGGNSTSLKVLDIQTGDTLKTLDTTPLSTITYIKQLYRESKFSKAQADLIRNIKTPLALGIQNSCQVIIVDIYFNLREQFLSSNQLILQDITNYDYKHFFNNKTNNLVPYFILGGDQLFNGNSYKFEYPAGKHSSEGYLVEDRNGITQQNLKSKLQHQYPQQQQQQQQQQQQQQTNQFTQLDVTSIEYIESLRMIAIGYSIGTFQLFSSNNFKLYYCSPAREVGLHSSVSHLENKQSPVTNFLYQELEDDDTSSVSHLWIGRGSKNNKSSNNNISIILYKLEFDLQLSPDSSKTINNLISLTQNVDTPIDITKINQTNSQTNQFGEILLMSYLYQNKDLKLNNGIIPKSKSIFIYQFIENGTIKIEIKLFDLFLLERHGINYSSNSQQHWLHSIKLDDENGNFKNNGYHSIWIDQQSVLNNVLYQLENNNSKVFLSKEDQYQTSGSNSGSGSDNFDDNYENFEENKLNLTIYHPNFKFKLLSFSTIDNIDYLSPKERLVYELSNKGAILFESSTLLNSVYVKFVESNIFPFYKSDQQQQRNDLLIFSLNNNLISIVKDYILNYKSSNAKLILESFWSHFQTLNRNFGLSEIYSKLNSDTPKLLELVYVKITDLVRIFKSLADRYIQENLNKLNSNDMIIDGGGGGGGSNSNSNLNSNSNLLPDTLKIKIDQAINIARFIEILKWSLYFGLFKPSTLNDMESVRNYTIQKRKIIKEKLTIEMGNIGRTNQYLSDRLLIDLFYSNIDLSSSTSTTTTTTTTTTDGNQIMSSYPPHNSQTMKSFFKIFESSQQFTKKISVLFYLLIDLELTDLNGGNGSNGKSLHQSETLKSFFGSFHISSNYYSFIMGIWKLDSYLLKSQDQMNIDDDDDDDEDATNRENNSNLIDEDIKSAFTLLNSSKVTKKYLYPILARFYSFGFKNYAQLLMKGFNFQPQTPDEAQLYVRILLSNHSILEAILFQRSFRNRLQDQLTIDSIERLLFSIFNYTFNLKKLDLILNMSLDEIEEQVFLHFLFKMKASSLISLYYIKRGRIPEACKVNRYYQSTRVNGDVFDGHDTINHLLLNYEQSLPLIQRPIHFNITNESQDKPKQQPQSQQQQQQPQPQQFLNSEEDNIPLLPKSISKVNLVPPQSFIQKPIVMPSPIPKLYNDSLYLSSTLSTAPISNLEILTKKSNEEQQERLLIQQRLAQQEKELQEQQRIKKEFEDQQEKLLDFQRQQELLQHQMEVHSQLLLQQKQQQQQQQKQIKEQEYEEYDEEYEEEEEEQVATSNKSSLDMIFPTMVTTTSTTTSSPNLSVASGSTPQGSPLKSALKSGGSAKKTTNVRFKDSLNREYPIPKLKKRGMPDSDDDDDDDDENYDSDDDDDDDEDSEFEDIYKIDSNEDEEEDEEDEEEEDDDSAVVHDDDELDDQQASQAQQFLQNQKHQKLLQQQQQQQQQQQQQQQQQQQQQQQQQQQQQQQQHETDDTEEELEDDIVEEDDDSEEDRFKDFERPKHGGKEPPKFSTYSGLQPSKQQQQKFLSPQDDDDYDEEDEEDDQSYDDDDDGEEEDDGNYRVPTQQFMRQPIVNSSSSGGTQDEPMEIGSSSDEDNSQIVKNQYNYNNEEDNDEDEQEDDNEEEQEEDEEEEEDSPKQPKRVVAHKPLPKVQFNNNDEEEQQQQQQQQQQQQQQQQQQQQQQQQQQQKEEEEEEEEEEEEKKMNESDESGGEISKNENSSDDDSDNDQFNSPFTNQFLSKTSGNTSGQSIDFDQDEKYSTPTDKGSNNNDTTVDSDIFQSQQSDSSFVQSQENESLKKSDENLSTFNDLNNSILSNISSQQPQEDDEKFQELEGDTNNNNNNNNNNNNNNNNNNNTDEVMGDEEKNDNQNVEMENTEQDKKDSPFQEIEDDESIINSQQKEESDVEGKSNDQSLETSIHQKVEDKQMDDDDDEKSNNQNEENVQPTQEKQDEQEPEEQEEQEKQPEEEEEEEEKVKEIEQQEEEEEEPKEEQSEEEEEEQPEEEQPEEEQTKEEQPGEEQPGEEEEEPEEEEEEKEPEEEEEEEKEMEEDEEEKEDEEEEKEDTPKKQPIVPISTRPSRQSKTDGIAKTLSIAEMRRGEKDKKKQLAPQKPTSKLKPKVQAATKPKKTKKASKK[4x];>MFGGQFGSFGAKPAATASPFGAPSAAPTTSLFGSTAPSSGFGGFGSTAQTTQPTTGGFGGFGGFGGATTTQQPAASPFGGGGTGGSGLFGSSAQTTTQQPGASPFGGGFGTTTTTTTQQPGASPFGGTGGGLFGSSAQTTTQQQGASPFGGFGGATTTQPSLLSGATGGFGGFGGSTTSGTQLGGGGGATSGAFGGSSSPFGGSGGATTSSPFGGGGGSFGATTQKQYGTPIPYQQTTIEGNTFVSISAMPQYNDRSFEELRFEDITHRKDIVYKTGGGSGGGNSLFGSTPTTQPSSPFGAQTTTQTTGGLFGGQTTTSPFGGQTSATPGSSLFGSTQPTQQQTSGGLFGSVQPTQQQAGGGLFGSMPSTGGSSLFGSTQPTQQQTGGAQPTQSLFGGQTQTTTSPFGSQTSTPFGQPQQTNTGSGLFGAQQTQQTNTGGGLFGAQPTQQTSGGGLFGTQPTSGTGLFGTSPTAGGTGLFGTTQPTSQGTGLFGTTQPTTQGTGLFGTSPTSGTGLFGSTPTSGTGLFGSTPTSGTGLFGSAQPPQNQQSQTSLFGNTGTGATNTGTGLFGSAQPSSNPGGGLFGSAQPSTTTGGLFGSNQPTAQPTTSLFGNTTGSVGGLGATPNITSGLFGSNPAQTGGLFGSTQPTTQTSLFGNTGSTGGLGAQNGGGLFGNLSQPTATAGQGLSGGLFGNLSQPTATAGQGLSSGGLFGNTLLGQPSTQGLSSALPTLGLGLMGGQPQQTQQLPQGSLMLQQTQQPLQQQPLQQQQQPLQQSTIQLNNQINSASPYFPISSPAPFATFVKDLTSTSKVVSPPSYTQRSLSHHGYIPKSTTKLVPRRGPNNVDLGFSVIQNQNGLFPIDKFITKHSKSLNINTTNETEDTLRSLNTKSSSLFNNNNNNNNNNNNRNVNTNVNDYQNNGLPSSSLYNSNINQLSNNNNNNNNIYNNNNNNNINNNNNNNNISTQFNLRNNQSSSDNLNNDKSLSSSSSNKSQQQQQKEQKEEQPPKPIKEKEFINPNAPKLTRDGYQCVPSIKELSKKTDKELSSVQGFTISRDGCGSIYFPGSTNLVALDLDDIVDIEPREVSVYKDEETKPEIGYGLNRDAVVTLENCWPKNKNGEVVKEDGTILDKYENALKKVSAKSDCGFVSYSRSNGTWVFTVKHF[4x];>[2x]MESQDIDYLKFNDFKSDIEDFEIGQDISGYDNSKIDFDSNVITISNEYGILLIVSPELNDLLVTPIEGLLNYIQSNDQDTNDQTTILSCPTIIKVGKVFEIPSSTKTSFKINLLFSPNGDYFSISYHKTLKVYSTKDSISKKWVNIKPIVEINGKFDSNIASTKWNHSNDTIAVVTANSSLFFVSIGNGSLNKIEEPAVDVCWDVKKSKQIYVALEDSSIILIDSSKPGHEIFRIENPITNYEDEDEEEEELNYYVSSINLVADEFLLVQYYIVRMDEYEDSPAFLFDLKDDESKSQEFQLSIMPEGNFQSAIHLASSFIKDWNLLIVCSNKGMGPDLLQLDTKTREWKTLKLEDEFGITLPNPVVLGMQLITCYPTQPKNLNGIQKYTTNGTFPPVPILLIVDDSAHFKFSNLFNINSKNLSIIQSPKSIQQQQQQQQQEQQQQQQTPSLFQSQTPSLFQQQKPQQPSSSLFQTTQTPAPSLFQQPQQTPTTSIFQQPKAPTTSIFQQQQQAPTTSIFQQQQQSPTTSILQQQQAPTTSIFQQQQQQQQSTQQQQKPKTIPTISPIKSMSTTFTNSVSTAPSQKQQQPSQQPSQQQQSQQQPFKRQNSAPTPISTPISTPIKNELSGNSNVYPNSTLKKYMQKIENTSNVYNGQSPISQQIRKNLKSIENYYQAIRRNSIEGNKIHQTIKNGFLANHQNTKTEIEEFQQSINSLTTEFKKNDKQSSLLKSQVLKNLSLSLDLESHTQQYSSTNYKQILANRNLDPSTLEQKDKLLSNYRNLSLDIQNFEQTHFKFLENNQNNQNNQNNIEKVHINSMSLIYQSLSNISQTETNLRCEIEKIEKKLNKLKLNKDKMDRLKDSIDINQYTELQLSRLSLENNVNILNDNGSGKDIKSTTKPTIENYRHEVNVSKSNGYKNLISVLKRKSSQVIKPQYPDFTSFFKSEQIDDPQFDDDIINNEYNNNNNNNSEIIEPPPALRGISLSKDNAFANSSYKFTSNITPIKTSGTISSPSSTTSSFTPTSHISFASTAQNFINNNQSYDDYQDGNEEYDEDDDDDDEQYDEDDEEYIEEPINPIPSLNKQQPQQQQQFGNNNNFGNLFNSQQPTNSNSLFTKNLDLEKEAKERQEKIERETRELQDKLEREEREAKEKQARELKDKLEREAKEKQARELKEKQEREAKEKAEKEANEKQEREAKEKAEKEAREKIEKEAKEKLEREAKEKLEREAKEKAEKEAKEKLEKEAKEKLEKEAKEKAEKDSANANNALGALNFGGNTTSTASGSSPFGSGGLFGTTTTPTTTAATPTPPSVFGGNSASTTTGGGSIFSQASTNSPPSPFGGSVFGAKPAPQTSSVFGSAPSTASAFGGSTTTSSFGATTATPTPFGGGGSVFGAKPAPQTSSVFGSTSSPSTTTSAFGSTSTTPSVFGNTSAFGGGGSTTTPTTSAFGSSSTTPAFGGTPAFGSAPTTSAFGSAPTTTTSAFGSSSTPAFGGTSAFGSAPTTSAFGSTPATGAFGSAPTTSAFGSTPATSAFGSTPTTGAFGSTPTTGAFGSTPTTSAFGSTPTTGAFGSTPTTSAFGSTSAFGSTPTTSAFGGAPTTNAFGSSSTPAFGSTPTTSAFGSSSTPAFGGTSAFGGAPTTSAFGSSSTPAFGGTSAFGSTPTTSAFGGGSVFGSTSSQPTSSVFGSQFGSNSAPSFASLGGGSFGK;>[2x]MKIREIIPLLSSNPLFSKTPQSSQKPSSFTSENNELSFTAKNFLSVNNQSSEIYYYSPIECKLYVIKVESTLDNTICAIRFQELKLKINFEVYKIELNEDSRYLCISGHVNCIIVDLNPQTVNSYFTSQEIFSDQENKTFGYDSLTVRSFTLDKTFYQSQISNIIKQVEWHPLSNIHLVILYSNNTLKIYNIQSGNEEIEQTFNLESIHTFESLKNLKNNDIRNQTKNTKKFISFCFGSNINFWTRFTIFLLSDSGEIFNLCPVIPNNCLVETSFYRDFQNHILYEKNQIENNSGSGSSNGDDSDEFIKQQQQQKKYYDFQFKWLMAASINTIPFEIENVSWLKLSSPSNSSTTFNPLLQGPISRISDSLPPSSNRVPLKILSIQPLVSNIDQNSNSSIINKINNNNNNDDDDNNNNNNNNNNNNNNNNNNDNDNDDDEKKKHNLSLSSTNKLIPFVIIVLMESCESLVNICCQDTIPMWSNDNGILYLEENNSNSNSKKQQQQQQQQQQPKYIDLILYEILDLNVKKSIKPSFSNIDKNLKNKSTIAIASTNQTKDYLSYSLPTMKYDQWSDSLYFYHNQGVQIAKFPWLYQIYLEINNIVAFENNNNNNNNNNNNNKNNINNSSTTNNNNNKNKNKNDEIDENIEFETTSLMSVINNGSGNGDQCIPIIGIQVFSNIKIGTYFLILPNTFKIIIFDMDGLINQQPNLHEQKQQQQQNDDNDDDDDDDDNDEDEINLKSPIQPFIDNPPSFIGRIILPNSFTQKEFLQTLVNTKKKLYNLYIYSNQLEIELNSRVKGLELISKDQLKLIDKLKIYIENLKSNQQALNAKLKYVWDKKEIDSEEIKELYKVEMEGKPLSNQEKELAKTLKQINSQVNIYSERLNQVEKDLQENNNNNNNNNNNNSSNINNNNNNNGLISVTSYETIPIEHQTEIKKVLNLHGQKIEEDVTKLEKLLKNIQI;>MDEEIFDNPIQKLNYNIRTEESGSLLKYLQSQKSNFTDSKKFISFKQKGNDSVGIRKEITQKKSFPLDNGFIGTVADPFIAIAFQISDRFNIDEYLACRILYSVVDHSTTRDEKELIELSEKFIYQNRSCYLQFLREILHTLQSRDSVNDINHSKMKHDILQSFIGELISEQTNDKNIVTILIKTLEEKVKDMNGTVNPLECCFRVKECIQIVECLFLISIQFTIKEDIIKLYIRVLNQVIEKEKREDSILKKSLFEIMFTLYFTIFAVFDNVKNSQVFNAIEKRYTFNEISSTDSIENEIKQIDNQHPIKSSLYAIFNIILIAKENNNSNSNSNSNSNSNSNSNNNNNRITPENDSYKFLLQAVQTQEYQLSPLNILFGSFINILSCRFLSNLSSHPTKKDILY[4x]FAN1 (FANCD2-FANCI-associated nuclease 1) is a DNA structure-dependent nuclease ubiquitously expressed in the central nervous system and peripheral tissues that plays a role in resolving interstrand crosslinks at replication forks. It possesses both 5′ flap endonuclease and 5′-3′ exonuclease activities, allowing it to process DNA structures that arise during replication stress and repair pathways. FAN1 comprises a DNA-binding SAF-A/B, Acinus and PIAS (SAP) domain, a tetratricopeptide repeat (TPR) domain that mediates dimerization and protein-protein interactions, a virus-type replication-repair nuclease module (VRR) containing the catalytic site, and an unstructured N-terminal region5. PCNA is a homotrimeric ring-shaped DNA clamp that encircles double-stranded DNA after being loaded by replication factor C (RFC).

To elucidate the impact of the HD-associated R507H mutation in FAN1, we generated a full-length recombinant FAN1 protein bearing the R507H mutation and reconstituted the ternary complex with PCNA and 5′ flap double-stranded DNA substrate. Although the overall conformation of FAN1 and the angle of the DNA substrate remained unchanged between the FAN1–PCNA–DNA and FAN1 R507H–PCNA–DNA complexes, notable conformational alterations were observed in PCNA. Specifically, the R507H mutation resulted in an increased distance of 16.5 Å between H507 of FAN1 and D232 of PCNA. This shift may allow for the observed interaction between H485 of FAN1 and Y211 of PCNA, a residue previously shown to play a critical role in modulating PCNA function. In the mutant FAN1 R507H–PCNA–DNA complex, H507 of FAN1 remains distant from D232 of PCNA (right). Furthermore, when the FAN1 R507 residue was mutated to H507, the interaction between PCNA D232 and FAN1 H507 was disrupted as evident by the increase in distance between these residues in FAN1 R507H–PCNA–DNA complex. Structural comparisons between the FAN1–PCNA–DNA and FAN1 R507H–PCNA–DNA complexes reveal a slight shift in the alignment between PCNA and FAN1, suggesting a compensatory effect at the PCNA-FAN1 interface. This shift facilitates an interaction between H485 of FAN1 and Y211 of PCNA.

> GPMGMMSEGKPPDKKRPRRSLSISKNKKKASNSIISCFNNAPPAKLACPVCSKMVPRYDLNRHLDEMCANNDFVQVDPGQVGLINSNVSMVDLTSVTLEDVTPKKSPPPKTNLTPGQSDSAKREVKQKISPYFKSNDVVCKNQDELRNRSVKVICLGSLASKLSRKYVKAKKSIDKDEEFAGSSPQSSKSTVVKSLIDNSSEIEDEDQILENSSQKENVFKCDSLKEECIPEHMVRGSKIMEAESQKATRECEKSALTPGFSDNAIMLFSPDFTLRNTLKSTSEDSLVKQECIKEVVEKREACHCEEVKMTVASEAKIQLSDSEAKSHSSADDASAWSNIQEAPLQDDSCLNNDIPHSIPLEQGSSCNGPGQTTGHPYYLRSFLVVLKTVLENEDDMLLFDEQEKGIVTKFYQLSATGQKLYVRLFQRKLSWIKMTKLEYEEIALDLTPVIEELTNAGFLQTESELQELSEVLELLSAPELKSLAKTFHLVNPNGQKQQLVDAFLKLAKQHSVCTWGKNKPGIGAVILKRAKALAGQSVRICKGPRAVFSRILLLFSLTDSMEDEDAACGGQGQLSTVLLVNLGRMEFPSYTINRKTHIFQDRDDLIRYAAATHMLSDISSAMANGNWEEAKELAQCAKRDWNRLKNHPSLRCHEDLPLFLRCFTVGWIYTRILSRFVEILQRLHMYEEAVRELESLLSQRIYCPDSRGRWWDRLALNLHQHLKRLEPTIKCITEGLADPEVRTGHRLSLYQRAVRLRESPSCKKFKHLFQQLPEMAVQDVKHVTITGRLCPQRGMCKSVFVMEAGEAADPTTVLCSVEELALAHYRRSGFDQGIHGEGSTFSTLYGLLLWDIIFMDGIPDVFRNACQAFPLDLCTDSFFTSRRPALEARLQLIHDAPEESLRAWVAATWHEQEGRVASLVSWDRFTSLQQAQDLVSCLGGPVLSGVCRHLAADFRHCRGGLPDLVVWNSQSRHFKLVEVKGPNDRLSHKQMIWLAELQKLGAEVEVCHVVAVGAKSQSLS;>[3x]GPMFEARLVQGSILKKVLEALKDLINEACWDISSSGVNLQSMDSSHVSLVQLTLRSEGFDTYRCDRNLAMGVNLTSMSKILKCAGNEDIITLRAEDNADTLALVFEAPNQEKVSDYEMKLMDLDVEQLGIPEQEYSCVVKMPSGEFARICRDLSHIGDAVVISCAKDGVKFSASGELGNGNIKLSQTSNVDKEEEAVTIEMNEPVQLTFALRYLNFFTKATPLSSTVTLSMSADVPLVVEYKIADMGHLKYYLAPKIEDEEGS Here, we report the crystal structure of the Lit enzyme from Bacillus cereus and describe its mechanism of action. Lit consists of four transmembrane helices with an extracellular cap. Conserved residues map to the cap-membrane interface. They include two catalytic histidines that function to effect unimolecular transacylation. The reaction involves acyl transfer from the sn-2 position of the glyceryl moiety to the amino group on the N-terminal cysteine of the substrate via an 8-membered ring intermediate.

The His85Ala and His85Arg mutants were chosen for complex formation since both were essentially inactive with this substrate. His85Ala and His85Arg were crystallised in the presence of the FP2 substrate and structures of both mutant forms were obtained. However, while density that could possibly be identified with the substrate was observed with the two mutants, it was not reliably fit with the lipopeptide as model. Our conclusion therefore is that the density observed in the substrate-binding pocket of these two constructs corresponds to structured monoolein molecules. In the His85Ala and His85Arg mutant structures obtained with crystals grown in the presence of the lipopeptide substrate, a different kink appears in M3 that causes it to curve away from M4. Curvature in M3 is such that it separates from M4 toward its extracellular end to a greater extent than seen in wild-type Lit. In so doing, it acts as a gate to create an opening between the two helices that leads into the putative active site. The fenestration extends into the dome providing a conduit at least 10 Å wide along its length presumably for both the polar peptide and apolar lipid parts of the lipopeptide substrate and product to move into and out of the binding pocket. The particular ‘open’ conformations captured in the inactive constructs likely reflect the fact that the catalytic residue, His85, has been mutated to non-conservative residues. Thus, while these mutant forms are not physiologically relevant, the structures they adopt may reveal features, such as the open gate, that are functionally relevant.

> MHHHHHHSSGRENLYFQGHMDRLITLVVSYSIAFSIFALATMAVVYGKWLYYFEIDFLNIPDLADMTKDEIKRNYDVLITYLSPFYDGALHLPTLDMSTNGRIRFVDVKNILVKIQYVMYATIMIAVIGGIYLLKKKNEKFLLHGSILTIIFPIALMLPIAINFEKSFVLFHKLLFSNDYWVFDPEKDPIILMLPEEFFMHAACAILLFILGGSILCYSLYRYLVKKKRMSQKKFSA>LEKFNVDLMKKAGKELGLSLSPNEIGCTIADLIQGQYPEIDSKLQRGDIITKFNGDALEGLPFQV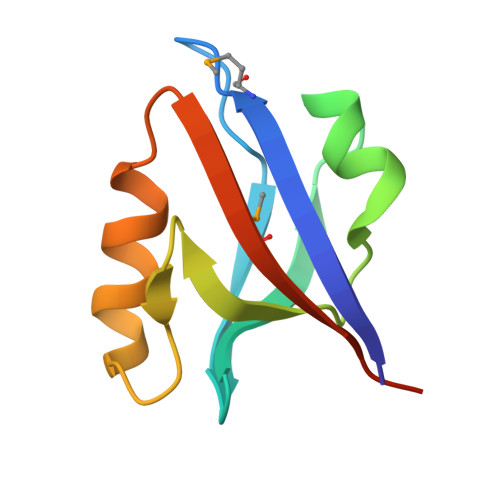CYALFKGANGKVSMEVTRPKPAAAS[3x]N-(2-hydroxy-1,1-dimethylethyl)-1-methyl-3-(1H-pyrrolo[2,3-b]pyridin-2-yl)-1H-indole-5-carboxamide | C21 H22 N4 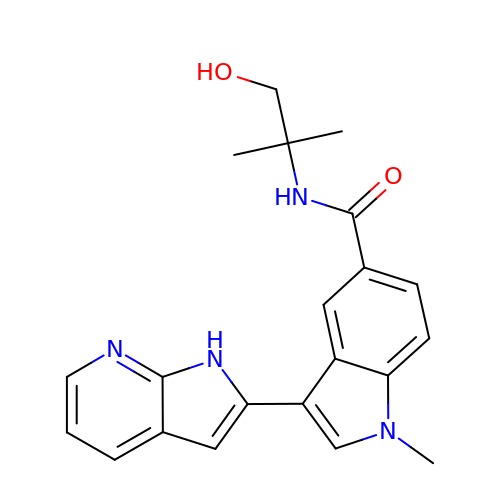O2 | XZRYCTLOGNCQDG-UHFFFAOYSA-N> AIAGAAGAUCUU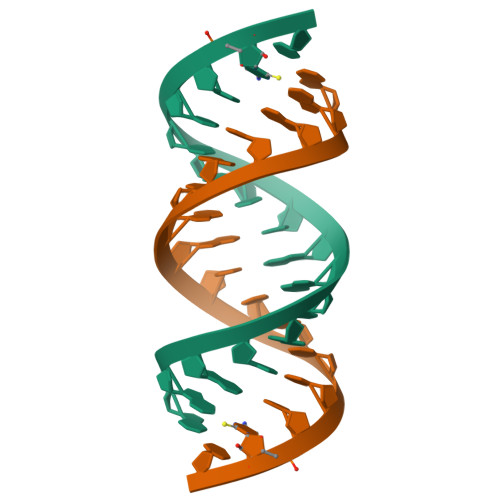CUCU> MPPQLHNGLDFSAKVIQGSLDSLPQEVRKFVEGNAQLCQPEYIHICDGSEEEYGRLLAHMQEEGVIRKLKKYDNCWLALTDPRDVARIESKTVIITQEQRDTVPIPKSGQSQLGRWMSEEDFEKAFNARFPGCMKGRTMYVIPFSMGPLGSPLAKIGIELTDSPYVVASMRIMTRMGTSVLEALGDGEFIKCLHSVGCPLPLKKPLVNNWACNPELTLIAHLPDRREIISFGSGYGGNSLLGKKCFALRIASRLAKEEGWLAEHMLILGITNPEGKKKYLAAAFPSACGKTNLAMMNPTLPGWKVECVGDDIAWMKFDAQGNLRAINPENGFFGVAPGTSVKTNPNAIKTIQKNTIFTNVAETSDGGVYWEGIDEPLAPGVTITSWKNKEWRPQDEEPCAHPNSRFCTPASQCPIIDPAWESPEGVPIEGIIFGGRRPAGVPLVYEALSWQHGVFVGAAMRS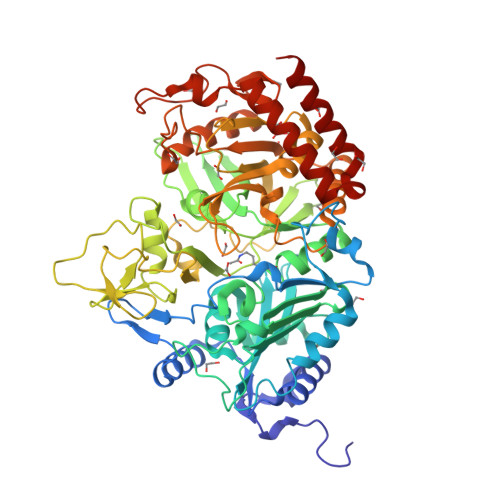EATAAAEHKGKVIMHDPFAMRPFFGYNFGKYLAHWLSMAHRPAAKLPKIFHVNWFRKDKNGKFLWPGFGENSRVLEWMFGRIEGEDSAKLTPIGYVPKEDALNLKGLGDVNVEELFGISKEFWEKEVEEIDKYLEDQVNADLPYEIERELRALKQRISQM7,8-DIHYDRO-7,7-DIMETHYL-6-HYDROXYPTERIN | C8 H11 N5 O2 | 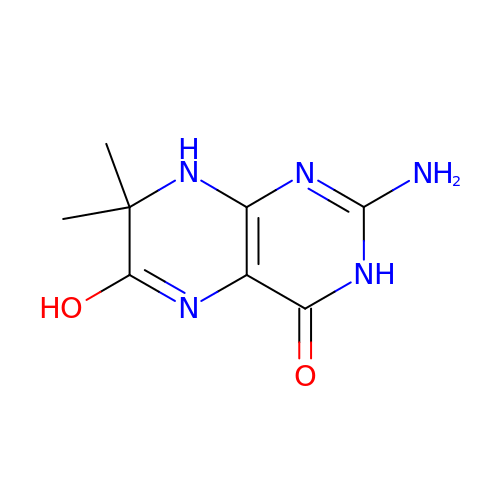JMLQSLXEUWNWFI-UHFFFAOYSA-N>MKINVPLESSNKTLSDLEKKKPFSVLLMGSDARAGEKNGRADTIILATANKQQNAVEMVSIPRDTKVDYGNGDIGKINASYSNGGPSGTVSAVEKLMPGVPVDYFISINMEGFKDLVDAVGGITVYNDIDLTEVNSKFVKGNITLNGTEALQYVRIRHEDPRGDFGRQDRQRDVIIGIANKVISSSGVSNFESIMKAVGDNFQTNMTLTDITSMAANYSSVLKNVDSQELKGEGEMIYSES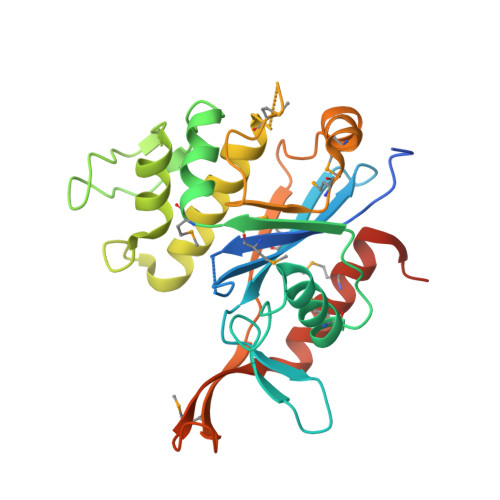YGFDLYYFAPDKTDLERIITMFKKSLDITELEHHHHHH[2x]> MVDGNYSVASNVMVPMRDGVRLAVDLYRPDADGPVPVLLVRNPYDKFDVFAWSTQSTNWLEFVRDGYAVVIQDTRGLFAS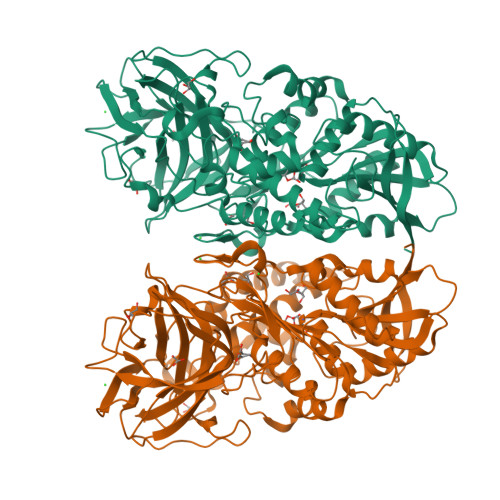EGEFVPHVDDEADAEDTLSWILEQAWCDGNVGMFGVSYLGVTQWQAAVSGVGGLKAIAPSMASADLYRAPWYGPGGALSVEALLGWSAKIGTQLITSRSDARPEDAADFVQLAAILNDVAGAASVTPLAEQPLLGRLIPWVIDQVVDHPDNDESWQSISLFERLGGLATPALITAGWYDGFVGESLRTFVAVKDNADARLVVGPWSHSNLTGRNADRKFGIAATYPIQEATTMHKAFFDRHLRGETDALAGVPKVRLFVMGIDEWRDETDWPLPDTAYTPFYLGGSGAANTSTGGGTLSTSISGTESADTYLYDPADPVPSLGGTLLFHNGDNGPADQRPIHDRDDVLCYSTEVLTDPVEVTGTVSARLFVSSSAVDTDFTAKLVDVFPDGRAIALCDGIVRMRYRETLVNPTLIEAGEIYEVAIDMLATSNVFLPGHRIMVQVSSSNFPKYDRNSNTGGVIAREQLEEMCTAVNRIHRGPEHPSHIVLPIIKRKLAAALEHHHHHH> MASHHHHHHGALEVLFQGPGYQMADEIDAMALYRAWQQLDNGSCAQIRRVSEPDELRDIPAFYRLVQPFGWENPRHQQALLRMVFCLSAG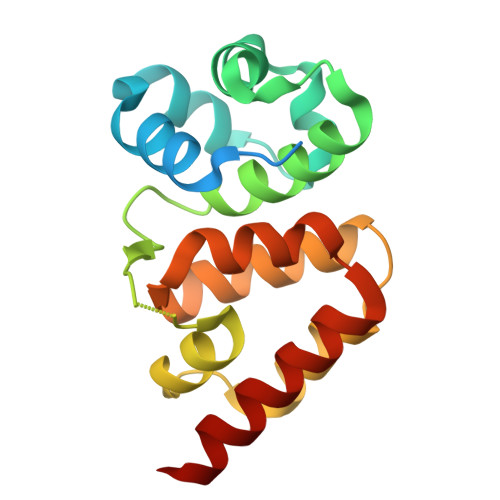KNVIRHQDKKSEQTTGISLGRALANSGRINERRIFQLIRADRTADMVQLRRLLTHAEPVLDWPLMARMLTWWGKRERQQLLEDFVLTTNKNA> TAQYSIIPEPSRTELRQETAKTLQLLSDQEVPTLETDAYRLTVTPQGAHLASGGREGRIYGLATLRQLRDQLAGQPEGIPCGVITDKPRYPWRGLMVDPARHFIPAADLKKFVDMMAYYKFNRLHLHLTDNQGWRLPVPGYPKLKSVASRREESFGDGIPHEGMYTKQELKELVAYCAARGIDVIPEIDMPGHNQALHAAYPEFFCFPKPDMNVRTTAGNSKELVCPQKPEVWKFYASVFNELKDIFPSGIVHLGGDEAPTELWEKCPLCREARTRAAMKDEQEQMKAFFAKTAALLAKNGQTPQFWYEGNAGIYHPGETVYAWRQGQALQSIEKTKKAGLNLIMASSEYCYLDFPQIQGQRNWGWMKTTTLQKCYDLDPAFGKPEKEAGHIRGVHAPVWAER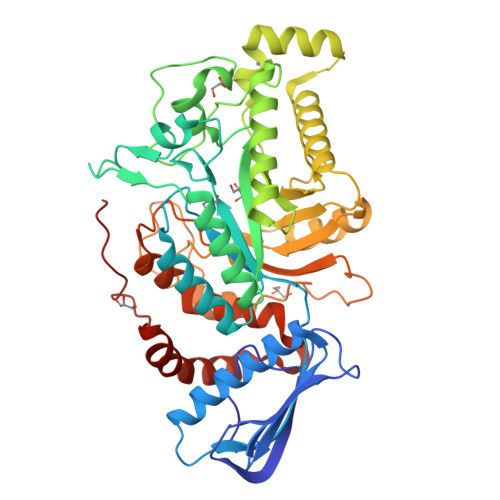LPDLNHLLYRAYPRACAIAEAGWSPMGVRSWENFRRKLADHRQFILKRFNYDMERTQGNEPAFRWE>[4x]VKLAGNSS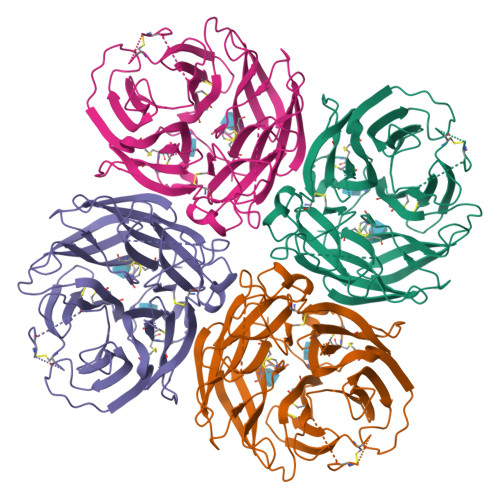LCPVSGWAPLSKDNSVRIGSKGDVFVIREPFISCSPLECRTFFLTQGALLNDKHSNGTIKDRSPYRTLMSVPIGSVPSPYNARFESIAWSASACHDGINWLTIGITGPDNGAVAILKYNGIITDTIKSWRNNILRTQESECACVNGSCFTVMTDGPSNGQASYKIFRIEKGKIVKSVEMNAPNYHYEECSCYPDSSEITCVCRDNWHGSNRPWVSFNQNLEYQIGYICSGIFGDNPRPNDKTGSCGPVSSNGANGVKGFSFKYGNGVWIGRTKSISSRNGFEMIWDPNGWTGTDNNFSIKQDIVGINEWSGYSGSFVMHPELTGLDCIVPCFWVELIRGRPKENTIWTSGSSISFCGVNSDTVGWSWPDGAELPFTIDK>[2x]GPLGSNISGQNTMNMVKVPECRLADELGGLWENSRFTDCCLCVAGQEFQAHKAILAARSPVFSAMFEHEMEESKKNRVEINDVEPEVFKEMMCFIYTGKAPNLDKMADDLLAAADKYAL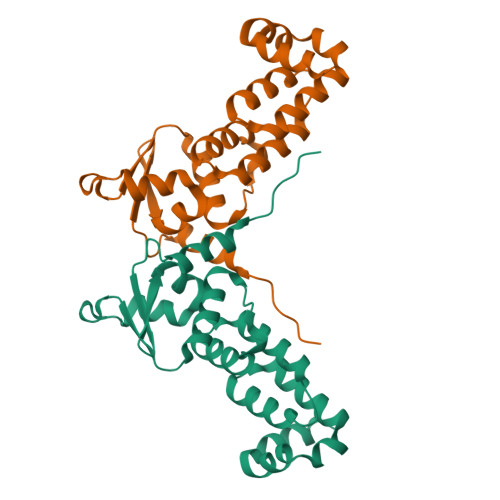ERLKVMCEDALCSNLSVENAAEILILADLHSADQLKTQAVDFINYHASDVLETSGWKSMVVSHPHLVAEAERSLASAQCPFLGPPRKRLKQS> GSALRELKVCLLGDTGVGKSSIMWRFVEDSFD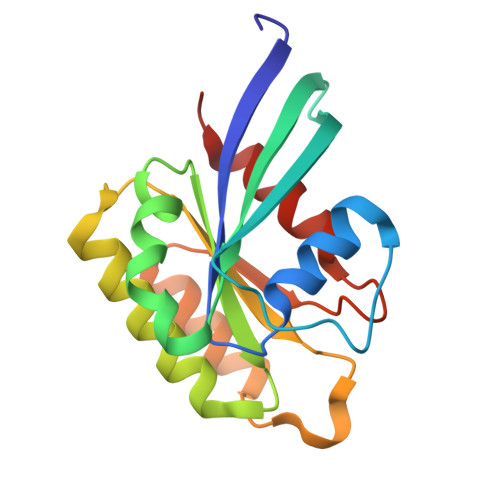PNINPTIGASFMTKTVQYQNELHKFLIWDTAGLERFRALAPMYYRGSAAAIIVYDITKEETFSTLKNWVRELRQHGPPSIVVAIAGNKCDLTDVREVMERDAKDYADSIHAIFVETSAKNAININELFIEISRRIPST> MKTIEQKIEQCRKWQKAARERAIARQREKLADPVWRESQYQKMRDTLDRRIAKQKERPPASKTRKSAVKIKSRGLKGRTPTAEERRIANALGALPCIACYMHGVISNEVSLHHIAGRTAPGCHKKQLPLCRWHHQHAAPAEVREKYPWLVPVHADGVVGGKKEFTLLNKSEMELLAD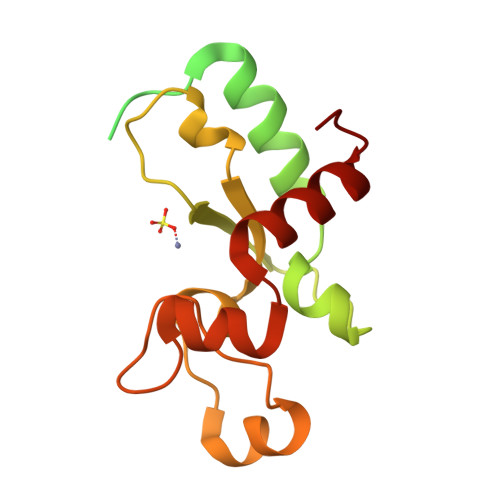AYEMANIMH>AQVINTFDGVADYLQTYHKLPDNYITKSEAQALGWVASKGNLCDVAPGKSIGGDIFSNREGKLPGKSGRTWREADIN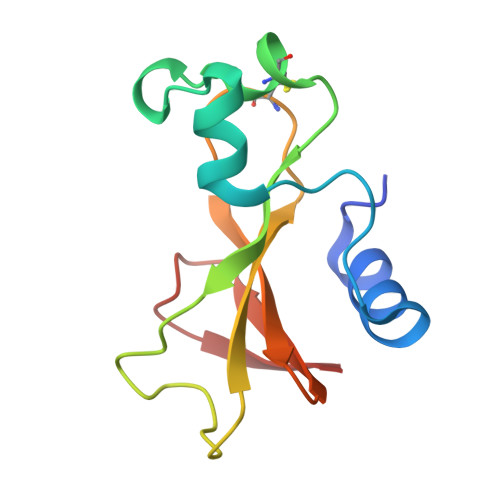YTCGFRNSDRILYSSDWLIYKTTDHYQTFTKIR[3x]> MNPIPAASDLKTRYPEFTGVSDAVVNAIIAEVNGMVDDGWEVSDQKPAVLALAAHMLSREGYPGRATNPNSFDPTNRPILSRKVGDVSTTFGR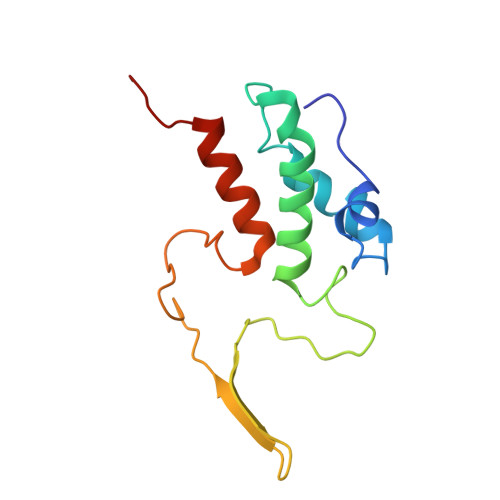TDGGAAEGGANSYNYSSTVYGQTFLRLLRLNAPAVGLV>[2x]GSMAVEVEVPTQVPAHIGIIMDGNGRWAKKRMQ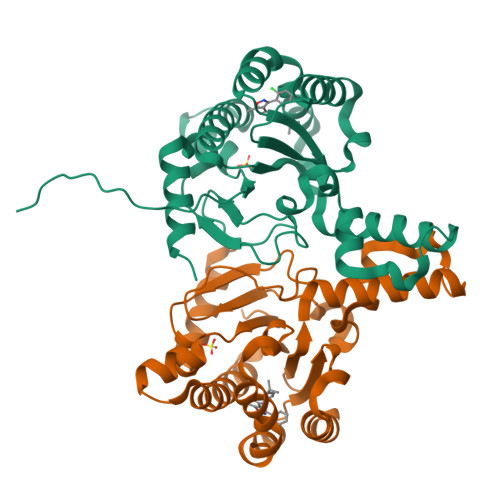PRVFGHKAGMEALQTVTKAANKLGVKVITVYAFSTENWTRPDQEVKFIMNLPVEFYDNYVPELHANNVKIQMIGETDRLPKQTFEALTKAEELTKNNTGLILNFALNYGGRAEITQALKLISQDVLDAKINPGDITEELIGNYLFTQHLPKDLRDPDLIIRTSGELRLSNFLPWQGAYSELYFTDTLWPDFDEAALQEAILAYNRRHRRFGGV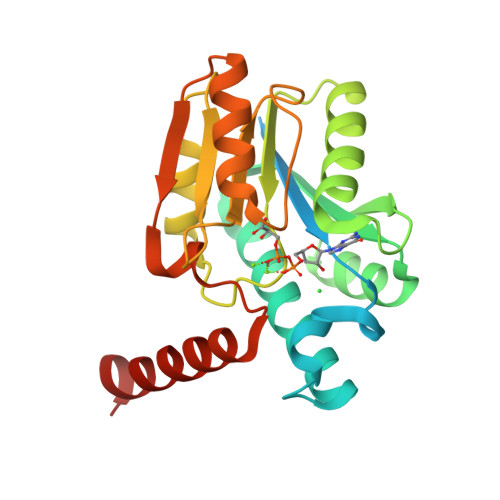>[2x]MGSSHHHHHHSQDPNSSSARLQVDKLAMSPVSVAQRNTGIWAVVPLKAPECAKTRLAGVLSHAARQALFFSMASHVIGTLRASPRIASLLVVTPSESTAEMARAAGAEILWGPPDEGMANACSRAMAHIAAAGGERVMFVPGDLPLLDEAAIDMLSRAPVDAIGMAPNRDGHGTNGLICRPGAIPLFFSGPSFSAHQNAARRAGIDVWVVRSREWALDVDLPADLEEFESSVRDAKRRVLCQN(2R,4S)-2,4,7-trihydroxyheptanoic acid | C7 H14 O5 | 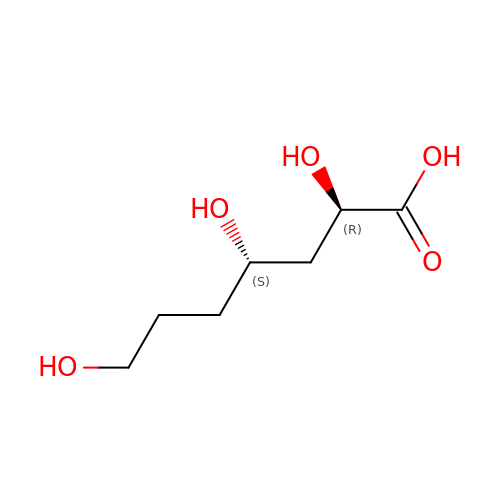UZWBQTOHZVUOKI-NTSWFWBYSA-N Many Gram-negative bacteria use a multi-protein type II secretion system (T2SS) to secrete a wide variety of exoproteins from the periplasm into the extra-cellular milieu. The T2SSs are composed of 12 to 15 different proteins that form three distinct subassemblies: (i) the inner membrane platform consisting of multiple copies each of GspC, GspF, GspL and GspM with an associated cytoplasmic secretion ATPase; (ii) the pseudopilus, a filamentous arrangement of multiple copies of five different pseudopilins; and (iii) a large, pore-forming outer membrane complex, mainly consisting of the secretin GspD. The inner membrane protein GspC consists of several domains: a short N-terminal cytoplasmic domain that is followed by the single transmembrane helix, a Pro-rich linker, the so-called homology region (HR) domain in the periplasm, a second linker and a C-terminal domain. Here, we studied the interaction between the outer membrane pore of the type II secretion system, the secretin GspD, and the inner membrane protein GspC.

The LBT to GspDN0-N1 facilitated crystal growth and the resultant crystals of the binary GspCHR–GspDN0-N1 complex diffracted to better than 2.7 Å resolution, with the LBT engaged in multiple crystal contacts. The structure of this binary GspCHR–GspDN0-N1 complex was solved by molecular replacement and refined with good crystallographic and stereochemical statistics. In the 2.63 Å resolution binary complex, the LBT introduced into GspDN0 faces away from the interface with GspC. The HR domain folds into a β-sandwich formed by six consecutive β-strands arranged as two three-stranded anti-parallel β-sheets. In its folded structure as seen in the complex with GspDN0-N1, the distribution of charges on the surface of GspCHR is quite uneven with the main hydrophobic surface interacting with GspDN0. The interface between GspCHR and GspDN0 buries 1280 Å2 of accessible surface area with a calculated ΔG of interaction of −5.4 kcal×mol−1 as assessed by the PISA server. A total of 18 residues from GspCHR and 19 residues from GspDN0 engage in a combination of hydrophobic interactions and hydrogen bonds. The first three β strands of GspCHR and the first β strand plus the subsequent helix α1 of GspDN0 are the major contributors to the interface. The majority of the hydrogen bonds are formed by an antiparallel arrangement of strand β1 of GspCHR and strand β1 of GspDN0. The interface and relative orientation of the N0 and N1 subdomains, however, is essentially the same in the two structures despite the binding of either Nb7 or the presence of the LBT insertion into the N0 domain: the superposition of the two N0 domains results in an r.m.s. deviation of 0.49 Å for 72 Cα pairs.

> GAMETRLNVVLRGIAFGARPGAVIEEGGKQQVYLQGERLDSHNAVIEEINRDHVMLRYQGKIERLSLA;> GAMAEEATFTANFKDTDLKSFIETVGANLNKTIIMGPGVQGKVSIRTMTPLNERQYYQLFLNLLEAQGYAVVPMYIDTNNDGYIEGDELVLKVVKSSAAKVEPLPLVGEGSDNYAGDEMVTKVVPVRNVSVRELAPILRQMIDSAGSGNVVNYDPSNVIMLTGRASVVERLTEVIQRVDHA> MPMLVVYVPEGYSEAQKRALLFRLAAAVVEATGTPLENVRIILTTYAPADVLLGG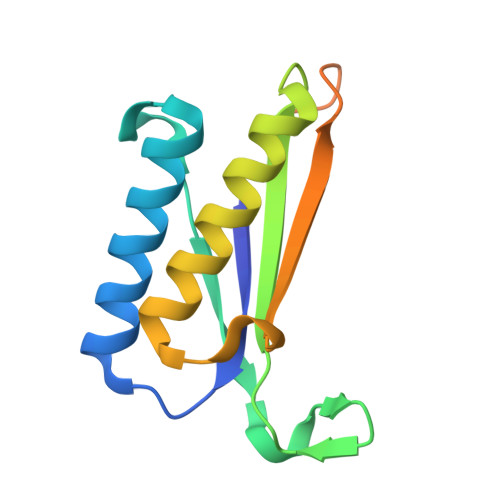AIGVPLVVILVYLLEGLSPEQKAALVKALTAAAAEALGVDPENIRVILVPVPPENFGVGNGKTAAEAGGSHHWGGHHHHHH>SNATDSPVLALAKELISRQSVTPADAGCQDLMIERLKALGFEIESMVFEDTTNFWARRGTQSPLFVFAGHTDVVPAGPLSQWHTPPFEPTVIDGFLHGRGAADMKGSLACMIVAVERFIAEHPDHQGSIGFLITSDEEGPFINGTVRVVETLMARNELIDMCIVGEPSSTLAVGDVVKNGRRGGGFLTDTGELLAAVVAAVEEVNHQAPALLTTGGTSDGRFIAQMGAQVVELGPVNATIHKVNECVRIADLEKLTDMYQKTLNHLLG[2x]

DapE hydrolyzes N-succinyl-L,L-diaminopimelic acid to L,L-diaminopimelic acid and succinate, is part of a biosynthetic pathway that is the major source of lysine in bacteria, and is essential for cell growth and proliferation. All the DapE enzymes characterized to date belong to the M20 family of dinuclear Zn(II)-dependent metalloproteases. In order to examine the role of the catalytic domain of DapE enzymes and the role of the active site loops, we have engineered the HiDapE and the DapE from Vibrio cholerae (VcDapE) by deleting their dimerization domains. Removal of the dimerization domain in DapE enzymes renders the enzyme inactive, even though the resulting truncated proteins have structures of the catalytic domain that are remarkably similar to WT-DapE and AAP.

Two VcDapET structures were determined, the apo- and the dinuclear Zn(II)-loaded form. The two V. cholerae structures are virtually identical and superimpose with the average rmsd of 0.25 Å for 265 equivalent Cα atoms suggesting that binding of Zn(II) does not induce any major structural changes. Likewise, the structure of Zn(II)-loaded VcDapET is almost identical to that of the catalytic domain of the full-length HiDapE with rmsd of 1.15 Å. The similarity between these structures is especially apparent within the active site region of Zn(II)-loaded VcDapET as the active site structure differs by only ∼0.45 Å rmsd with the active site of HiDapET and ∼0.4 Å with the WT-HiDapE. The active site of Zn(II)-loaded VcDapET contains a (μ-oxygen)(μ-carboxylato)dizinc(II) core with one terminal carboxylate and one histidine residue at each metal site ([ZnZn(VcDapET)]), that is identical to the active site observed for WT-HiDapE. Based on the best fit, an ethylene glycol molecule was modeled in the active site resulting in a distorted tetrahedral coordination geometry for Zn1, which is bound by the carboxylate oxygen atoms OD1 of D101 and OE1 of E164 as well as a nitrogen atom NE2 of H68. Zn2 adopts a distorted trigonal bipyramidal geometry and is coordinated by the bridging O2 oxygen atom from ethylene glycol, a nitrogen atom NE2 of H239, two oxygen atoms, OD2 from D101 and OE2 from E136, and the O1 oxygen atom of ethylene glycol. The Zn1-Zn2 distance is 3.39 Å. Identical to CPG2, HiDapE, and AAP each zinc ion is coordinated by one imidazole group (H68 for Zn1 and H239 for Zn2) and the oxygen atoms of E164 for Zn1 and E136 for Zn2. Both zinc ions are bridged by D101 and a single oxygen atom of ethylene glycol (in the molecule one, chain A) and a water molecule (in the second molecule, chain B).> FLPAAAPETDSLERMFLDALESGRIPEAQRMLSALGALRPSFENTAELEDLPLPATLAEGPGAPRLICVSTPTANGGVHEYARLAASFRGERHVSALPLVGFAAGERLPATPETAVRVVAESTLRASDGNPFVLVGHSSAGAFAYLAAALLENTWGIRPEAVVLLDTLSLRHEQNETIDYAGLMRRHFMVDEVSPVRMTNSRLSAMARWMGMLNQLEVRHTTVPVLIIRAAKETFGIGTDTGIYGEDHGS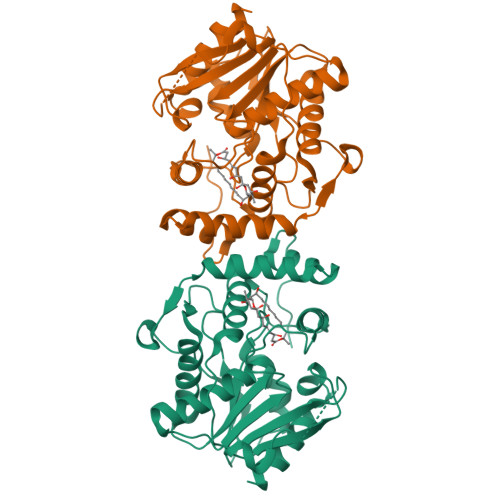PVDVRSVDADHFSMVRDDAPETARIVKEWLDSLGNA> VFGYVTEDGDTALHLAVIHQHEPFLDFLLGFSAGHEYLDLQNDLGQTALHLAAILGEASTVEKLYAAGAGVLVAERGGHTALHLACRVRAHTCACVLLQPRPSHPRDASDTYLTQSQDCTPDTSHAPAAVDSQPNPENEEEPRDEDWRLQLEAENYDGHTPLHVAVIHKDAEMVRLLRDAGA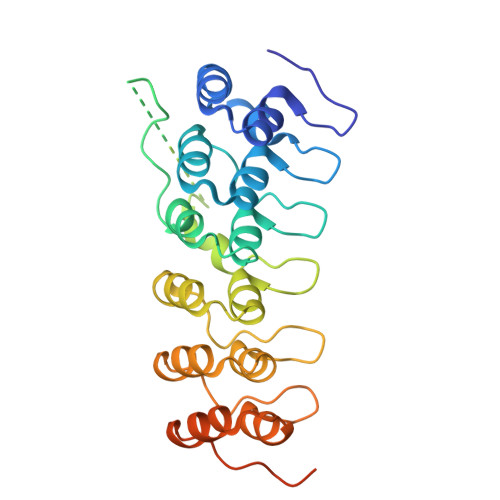DLNKPEPTCGRTPLHLAVEAQAASVLELLLKAGADPTARMYGGRTPLGSALLRPNPILARLLRAHGAPEPEDGGDKLSPCSSSGSDSDSDNRDEGDEYDD>DPEQLKWISFCLFLICL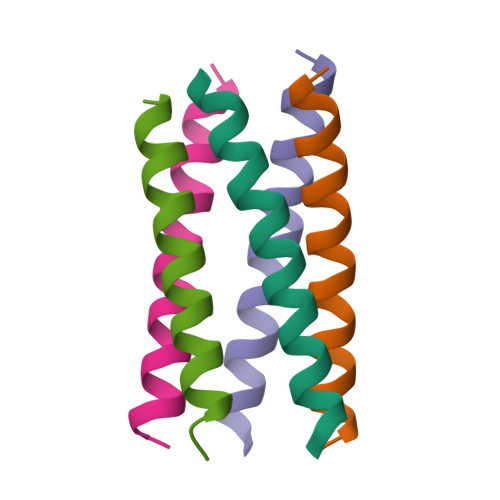LLLCIIFMLYRGRGSX[10x]> MGSSHHHHHHSSGENLYFQGSHMTA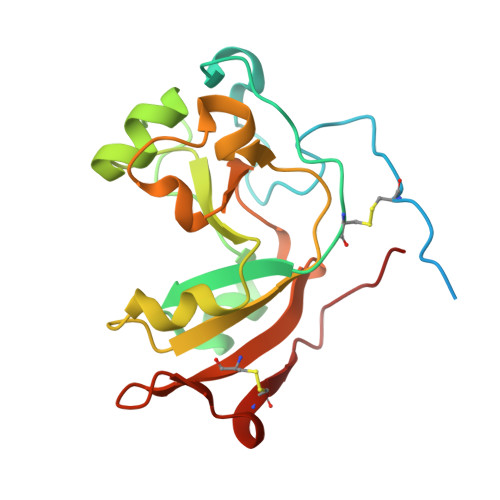TATSAKAAAPACPRFDDPVHAAADPRVDVERITPDPVWRTTCGTLYRSDSRGPAVVFEQGFLPKDVIDGQYDIESYVLVNQPSPYVSTTYDHDLYKTYYKSGYNYYIDAPGGVDVNKTIGDRHKWADQVEVAFPGGIRTEFVIGVCPVDKKTRTEKMSECVGNPHYEPWH> GSPRSYLLKELADLSQHLVRLLERLVRESERVVEVLE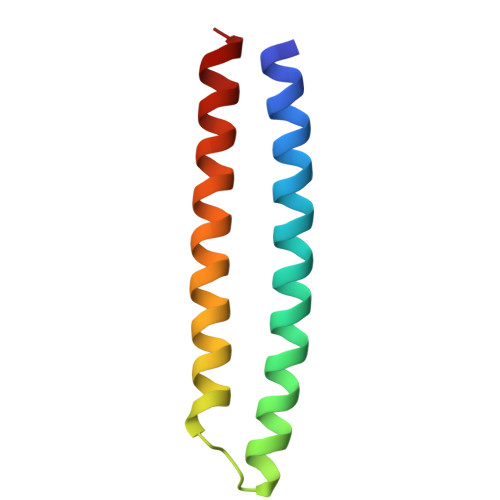RGEVDEEELKRLEDLHRELEKAVREVRETHREIRERSR Unlike the dissociated systems of individual enzymes that make up type II FAS systems in plants and bacteria, Type I FAS systems in fungi and animals are large complexes that integrate the key enzymatic activities required for fatty acid biosynthesis. In particular, yeast type I FASs are 2.6 MDa hetero-dodecameric complexes with an α6β6 configuration, which form a cage-like structure comprising two dome-shaped reaction chambers on either side of a central platform. Along with structural support regions, enzymatic domains form the walls of the reaction chambers, with most active sites facing the chamber interior. The mobile acyl-carrier protein (ACP) domain tethers the growing fatty acid chain and carries it between active sites, so each can act on this in turn.

Here, we report the 3.1-Å resolution solution structure of P. pastoris FAS, determined by cryoEM. Classes corresponding to FAS were taken forward and processed separately, yielding a 3.1 Å reconstruction from ~ 37,000 particles, with parts of the central platform resolved to ~ 2.7 Å. Density was present for most domains of the α- and β-subunits, including acetyl transferase (AT), ketoacyl reductase (KR), ketoacyl synthase (KS), enoylreductase (ER), dehydratase (DH) and malonyl/palmitoyl transferase (MPT) domains. The α subunit is mostly resolved, though several segments of the peptide sequence (including the ACP and PPT domains) are missing (residues 96–322, 535–598 and 1752–1879). The β subunit is practically complete, lacking only a small number of residues at the N- and C-termini (residues 1–9 and 2064–2069). We also observed density for a ligand bound within the active site of the ER domain (for reference), presumably a molecule of FMN. Visual inspection confirmed that several domains appeared shifted, particularly the MPT domain. Here, the ferredoxin-like subdomain is positioned further away from the α/β-hydrolase fold in P. pastoris FAS, opening up a cleft between the two subdomains close to the active site. In particular, Q171 was shifted within the active site of the AT domain. H749 of the ER domain was also pointing in the opposite direction to the equivalent histidine in S. cerevisiae FAS.

> MRPEVEQELSHVLLTELLAYQFASPVRWIETQDVFLKDYNTERVVEIGPSPTLAGMASRTIKAKYESYDAALSLQRQVLCYAKDTKEIYYTPDPADIAPPIKEEAETSAAATSSSAPAAAAPVSAAPAAAPSGPVAEIPDEPVKAALVLHVLVAHKLKKSLDAVPLSKAIKDLVGGKSTVQNEILGDLGKEFGSTPEKPEDTPLQELAEQFQDTFPGSLGKQTGSLVNRLMSSKMPGGFSLSVARKYLQTRWGLGPGRQDSVLLVALVNEPGARLSSDGEAKEFLDSCAQKYASGAGITLAQAAAGGAGSSGAGGAVIDAEAFEELTKDNRVLARQQLEVLARYLKYDLTKGEKSLVKEKEASSLLQQELDLWAEEHGEIYAQGIKPVFSHLKARTYDSYWNWARQDALSMYFDIIFGKLTDVDRETVSQCIQLMNRSNPTLIKFMQYHIDHCPEYKGETYQLAKSLGQQLIDNCIQVANQDPVYKDISYPTGPHTEVDSKGNIVYKEVNRKSVRKLEQYVFEMSQGGELTKEVQPTIQEDLAKIYEALNKQASTESQLEFNKLYNSLIEFVEKSKEIEVSKSINAVLASKSSDSDRSAEISSLSEKTSIVDPVSGGIPPETVPFLHLKKKLPSGEWVFDRDTSALFLDGLQKGAVNGISYKGKNVLITGAGAGSIGAEVLQGLISGGAKVIVTTSRFSKKVTEYYQDIYARFGAAGSCLIVVPFNQGSKQDVEALIDYIYRDVKDEGLGWDLDAVIPFAAIPEAGIEIDELGSKSELAHRIMLTNLLRLLGEVKKQKFTRAINTRPAQIILPLSPNHGTFGSDGLYSESKLGLETLFNRWYSESWSEQLTVCGAIIGWTRGTGLMSGNNIIAEGLEKLGVRTFSQKEMAFNILGLMTPELTEMCQNGPVVADLNGGLQFIENLREYTAQLRNEIYETSEVRRAVSIETGIETRVVNGENADAPYQKARIEPRANLKFEFPPLKSHKEIQNKAPGLEGLLDLERVIVVTGFGEVSPWGNTRTRWEMEAFGEFSIEGCLEMAWIMGFIKYHNGNLKGKPYTGWIDAKTNEPVEDKDIKKKYEEEILAHAGIRLIEPELFRGYNPEKKELIQEVIIEQDMAPFVTDESTAQQYKLQHEDAVDILKSEESDEYTVTFKKGARLFVPKALRFDRLVAGQIPTGWDAKRYGISEDTISQVDPVTLYALVSTIEALLSAGITDPYEFYKYVHVSEVGNCSGSGMGGVSALRGMFRDRYSDKPVQNDILQESFINTMSAWVNMLLLSSSGPIKTPVGACATAVESVDIGVETILSGKAKICLVGGYDDFQEEGSYEFANMNATSNSLDEFDHGRTPQEMSRPATTTRNGFMEAQGSGTQVIMNAELAIKMGVPIYAIVALTATATDKIGRSVPAPGKGILTTAREHHGSLKTKSPKLDIKYRTRQLNKRKDQIKQWVEDELEYIREEAAELANSDAKFDAVSFVSERTEEVYREATKQVKMAQQEWGNEFWKNDPRIAPLRGALATFNLTVDDLGVASFHGTSTKANDKNESITINKMMQHLGRSEGNPVFGVFQKYLTGHPKGAAGAWMLNGAIQILQTGIVPGNRNADNVDKILEDFEYVLYPSRSIQTDGIKACSVTSFGFGQKGGQAIVVHPDYLFASLDSETFEEYKTKVEARYKSTYRYMHNAIIRNTMFVAKSDPPYTDELEQPVYLDPLARVNNCKKNPSKLVFVNADVQSKQNFVGKSANDTAKVISSLTSDVTSGGKGVGVDVELISAINNENHTFIERNFTENEISYCASAPSSKSSLAGTWSAKEAVFKALGVESKGAGASLKDIEIVRDSKGAPTVVLHGDAKSAASAAGVKNVKVSISHDDVQSVAVAISEF;> MSATSGVVNRPLVLNHGSIESTILIPTTEYHFYQTLLEGFRKSLPQVTEGFADDDEPSSKAELLMKFLGYIVQSGVSNQQEQLAAAKLVLNEFESRFLQGLNLHSYAAILLKSETFPTTLLKIKENLIKNYYLGRALVYLPGQRGLVYPPSALLNAGKSGSAQIYAIFGGQGNTDDYFEELRDIYHIYQGLVSDFVTKAQLKLQELIRTTPETDRIYTQGLDLINWLENKDKTPDQQQLLSIPMSCPLICVIQLCHYIVTCRILGITPGQLRDSLKGTTGHSQGLVTAVVVSSADSWESFEKLALQAVEFMFYIGVRGLQTYPNTSLPPSIVQDSEENAEGTPSPMLSVRDLSYDQLVKFVNETNQHLPEAKHIDISLINGPRNVVLTGPPQSLYGLNLNLRKAKAPSGLDQARIPFSERKLRFSNRFLPIMSPFHSHLLSPSTEKIVADLKKAGVEFSQSSMKLPVFDTYDGKDLRSYSGSIAARLVECITKLRVNWELSTEFNSTHVLDFGPGGASGLGVLTHRNKEGTGSRVIVAGVLDAESEDSEFGYKQEIFESNEKAIKYAPNWLKEYKPKLVKTSAGKIFVDTKFSRLLGRAPLMVPGMTPTTVSPDFVAATLNAGFHTEIAGGGYFAPSIMKAALQRVIDQVTPGTGVGINLIYVNPRMLQWGIPMIKELREQGFPIQSLSIGAGVPSLEVATEYIETLGLAHLGLKPGSIDAVNQVITIAKAHPNFPIVLQWTGGRGGGHHSFEDFHQPILQMYSKIRKCKNIILIAGSGFGSAEDTYPYLTGSWSHQFSYPSMPFDGVLFGSRVMTAKEAKTSPAAKQAIADCTGVDNSQWENTYKKPTGGIITVRSEMGEPIHKIATRGVMLWKELDDTIFTLPKNKMLEAIAKKKDYIIKKLNADYQKPWFAKNEKGTCDLEDMTYKQIAERLVELMYVRKSQRWIDVTLRNFTGKFLRRIEERFATKVGTISLIQNFSQLEEPEKAIDSVFKAYPEAASQLINEEDCDWFLLEAQSPTQKPVPFIPVLDERFEFFFKKDSLWQSEDLEAVVGEDVQRTCILHGPVAAQFSNKVDEPIKDILENIHKGHIKSLVKEVYNGDESKIPVVEYFSSVDSFSDTAIEGVKIERSRNTETFTVTSGNVDNQQWFDLLAGKELSWRRAFITAARLVQGTNFVSNPAHSVLAPSKDLVVKIENGSDAKKTVLTAFQRVRGKYVPAVSLKSIGDLKIKLELIETRTADKSAVALELFYNYKPTDGFAPILEVMEGRNTSIKNFYWKLWFGSSVPVDLDFDANKPISGGEASVSSQAIAEFTHAVGNSCEDFVPRAGRPQLAPMDFAIVLGWKAIMKAIFPKTVDGDILKLVHLSNGYKMFPGADPLKKGDVVSTVAHIRSVVNGETGKTVEVVGVISRDGKPVLEVNSQFFYRGKYQDFGNSFKKTTETPVQVAFKSAKDIAVLKSKEWFHLEKDIDLLNQTLTFRCESYVKFKSSTVFASVKTTGQALLELPSKEIIQVAEINYESGSSYGNPVLDYLTRHGSTIEQPIMFENAIPLAQGTELTSKAPGTNETYAAVSGDYNPIHVNKVFASYANLPGTITHGMYSSAAVRALVEQWAAQNVATRVRAFKADFVGMVLPNDELVTHLEHVGMINGRKIIKVETKKVETEEVVLIGEAEIEQPVSTFVFTGQGSQEQGMGMDLYNSSEVAKSVWDRADVHFINNYGFSILDIVKNNPTELTVHFGGAKGRSIRNNYISMMFETVAADGQLKSEKIFKEINEDTISFTFKSPTGLLSATQFTQPALTLMEKASFEDMKSKGLVPSESMFAGHSLGEYSALTSLGDVMPIESLVDVVFYRGMTMQVAVPRDEQGRSNYGMIAVNPSRVSSTFNDSALRFVVEHIAQQTGWLLEIVNYNVENTQYVAAGDLRGLDTLSNVLNVFKIQKIDIVKLQETISLDEVKVHLSEIVDEVSKKSSSKPQPIDLERGFACIPLKGISVPFHSSYLRSGVKPFQTFLCKKIPKSAVKPANLIGKYIPNLTAKPFQLTKEYFEDVYELTKSEKIKHILDHWEEYESS> HKVIKNETGTISISQLNKNVWVHTELGYFSGEAVPSNGLVLNTSKGLVLVDSSWDDKLTKELIEMVEKKFKKRVTDVIITHAHADRIGGMKTLKERGIKAHSTALTAELAKKNGYEEPLGDLQSVTNLKFGNMKVETFYPGKGHTEDNIVVWLPQYQILAGGCLVKSASSKDLGNVADAYVNEWSTSIENVLKRYGNINLVVPGHGEVGDRGLLLHTLDLLK

The production of β-lactamase enzymes, which catalyze the hydrolysis of the endocyclic amide bond of the β-lactam ring, is the most common mechanism for resistance to these antibiotics. Class B enzymes are zinc dependent metallo-β-lactamases (MBLs), which require one or two Zn2+ in their active site for catalysis. Note, the 5/B/6 MBL, which we use in our biochemical and structural studies, is a different isolate from the commonly used BcII MBL (Sequence ID: EEL64219.1). In this paper, we couple kinetic and structural studies of the free and inhibited Bacillus cereus 5/B/6 MBL to understand the structure-activity relationships that underlie the inhibition by the 10-mer DNA.

To put the mechanism of inhibition into a structural context, X-ray crystallography trials were initiated for the aptamer-free and 10-mer-bound enzyme. The 2.5 Ångström (Å) resolution crystal structure of aptamer-free 5/B/6 MBL with both Zn2+ ions bound is shown in Fig 2. Subclass B1 MBLs display a αβ/βα sandwich fold in their tertiary structures with a consensus sequence of HXHXD(X)iH(X)jC(X)kH (in single letter code for amino acids where X = any amino acid, i = 55–74, j = 18–24, and k = 37–41), with H, D, and C residues coordinating the Zn2+ ions. Our structure shows a similar fold. Interestingly, our structure shows that in 5/B/6 MBL Zn2 has a higher B-factor compared to Zn1, indicating that Zn2 exhibits a partial occupancy in the active site pocket unlike Zn1. Coupled to this, the active site residue His263 is found to be in two conformations in the X-ray structure. This result suggests that His263 plays an important role in directing Zn2 to its location within the active site by acting as a gate locking Zn2 in place once it is bound. Interestingly, all of these residues are on the opposite side of the enzyme from the active site in three structurally adjacent loops (L4, L6, L13). Among these residues were three lysines (78, 104, and 107) on loops L4 and L6, shown in the crystal structure in Fig 2A, that make up a basic patch. The side chain amines of Lys78 and Lys107 are 11.7 Å away from each other providing ample space to occupy the loop region of the 10-mer (~8.7 Å distance between A5 and C6 of the aptamer). The shortest distance between the active site and inhibitor binding site is 25 Å, as measured from His116 to Lys78 –too far away for the aptamer to interact directly with both sites. 200 models of the complex were calculated using our X-ray crystallography model and a hairpin model of the 10-mer aptamer, which was calculated in 3D-NuS.[4-(2-hydroxyethyl)piperidin-1-yl](5-methyl-1H-indol-2-yl)methanone 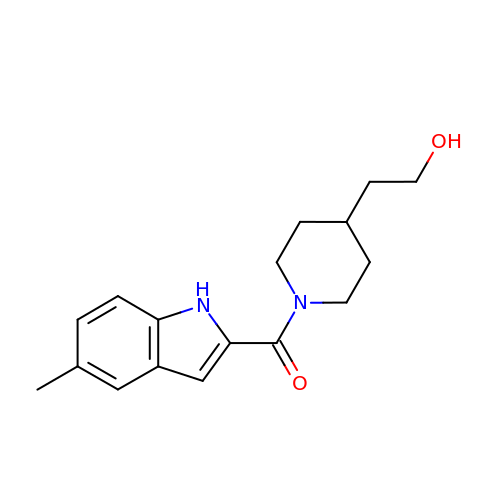| C17 H22 N2 O2 | HBSLSZOJAXYBQI-UHFFFAOYSA-N> MESGIDLQGQFISALQSLGLSHDLAKLLWLPLPMLMMLIVATVGVLVAVWLERKISAAVQQRIGPEYIGPLGILAPLADGLKLIFKEDVLPANSDRWLFTLGPAVVVIPVFLSYIIVPFGQNLLISNLAMGVFLWIALSSIAPIGLLMAGYASNNKYSLLGGLRAAAQSISYEIPLALAVLAVAMMSNGLGTVEIVEQQSQYGILSWNVWRQPIGFLVFWIAALAECERLPFDLPEAEEELVAGYQTEYAGMKFALFYLGAYVNLVLSALLVSVLYFGGWSFPIPLETIANLLGVSETNPFLQIAFAVLGITMTLIKAYFFVFLAILLRWTVPRVRIDQLLDLGWKFLLPVGLVNLLLTAGLKLAFPVAFGG;> MDLVTLAGQLNAGTILPETILIVTLLVVLLADLIQGRQADRWTPYFAIVGLGGAIATMIPLWTQPATISFFGSFISDHLSLFFRGLIALSALGTILMSIRYVEQTGSSLGEFMTILLTATVGGMFIAGAQELVFIFVALETLSIASYLLTGYTKRDSRSNEAALKYLLIGAASSAIFLYGSSLLYGLSGGHTQLPAIAQALSSESLGLVVALVFVIAGISFKISAVPFHQWTPDVYEGAPTPVVAFLSVGSKAAGFALAIRFLTLAFPSVTDQWQLIFTVLAILSMILGNVVALAQTSMKRMLAYSSIGQAGFVMIGFVVGTEAGYASMLFYLLVYLFMNLGAFTCVILFSLRTGTDQISEYAGLYQKDPLLTLGLSLCLLSLGGIPPLAGFFGKIYLFWAGWQAGAYGLVLLGLLTSVISIYYYIRVVKMMVVKEPQEMSEAVRNYPEVSWSSFGLRPLQVGLVMTVIATSLAGILANPLFNLVNTAVWDVPQLANQPTVMEVAYQALSPAGKS;> MVAIPRLRDTATVFVLSGYEYFLGFLIICSLVPVLALAASALLRPKSGRMIRLTTYESGMEPIGGAWIQFNVRYYMFALVFVIFDVETVFLYPWAVAFHQLGLLAFIEALIFIAILVVALVYAWRKRALEWS;> MLHSLRFLPMLTLLIVLPVIGALLMPLLPERVLRSVALVIAGLTFALSLWMLTQFDVHQSALQFTEFVPWLLPLGLNYSLGVDGLSLPLIVLGTFLTLGVVFTGEKTGQRLFYALVLLANAGITGALAAQNLLLFFLFYELELVPFYLLILIWGGQRREQAAVKFLIYTAVSGILVLAAFLAMGWLTHAPSFDSADIQIAGLAPTTQGILLLLLILGFGIKMPLVPLHSWLPDAYVEASTPTAILLGGALAKLGAYGLVRFALGYFPEAWAQFSGLLAIVAAVGIAYGALAAIAQKDIKRMVAYSSIGHMSYVLLAAAAHTHLSMVGAIAQMISHGLILALLFYLVGVIETKVGTRELNVLNGLLNPLRGLPTTSALLILGGMASAGIPGLVGFVAEFLIFQGSYGMFPLPTLVAVVGTGLTAVYFVIMINRTCFGRLDNRTAYYPRVVWSEKMPALVLTLLIVFLGVQPTWLVRWSETTSAQIVAAVPRTNELVATLAKR;> MQLTYVLILAALLFCIGIYGLVTSRNAVRVLMSIELLLNAVNLNLIGFANYLDGQQIKGQVFAVFVITVAAAEAAVGLAIILAIYRNRDTVDMEKFNLLKW;> MLQSFADTVWLIPFYSLAGMVLSLIWSPGITRKTGPRPAGYLNILLTFFSFVHALLATVAIANQPPQYLHWTWLDVAGLHLDIPVEISILTTTALMLITALNLMAQVFAVGYMEMDWGWARFFALLALFEGGMGALVLLDSLFFNYVVLEILTLATYLLIGLWFNQPLVVTGARDAFLTKRVGDLVLLMGVLAIYPLAGSWNYDDLAAWAATAQVNSTLITLICLALIAGPMGKCAQFPLHLWLDEAMEGPIPASILRNAVVVATGAWVLVKLTPVLSLSPVALTALLVIGSVTALGGTLIAIAQVDIKRALSYLVSAYMGWVFIAVGLKEPGLAFVFILTYSLAMAVLMMSIGSIIWNSVTQDLRLLGGLWSRRPISGISFLVGSAGLLAVPPLASFFPQAELLDTAFAQLPWVGGVLLLMNTFAAFSLGRTFCLVWGGEVKPMTARSPEVFWPMILPMTVDLGLVLHLPILMARFDWVIWTQPSLATAAALTITALLGWGVAAWVYLGKAIPKPVQFPLPSVQNLLAYDFYTPKLYRATVVGVVDMISRITAWFDRTFVDGTGNAFGVVTLLGGDRLKYSTTGQSQAYILTILMGIAILVIAICWPLLA;> MDLATLTQTITFFALAAAVIIAALGVVLLDNVVYSAFLLGGVFLSIAGLYILMNADFVSAAQILIYVGAVNVLILFAIMLVNKRETYTPVPGRWLRQGGAAVVSLGVFALLTKMILQTPWQLSSVPPTPDSITTIGQHFFSDFLLPFELASVLLLMALIGAVVLARRELVLEPEPILGEEVVPPLELPERPREPVALSEK;> MPKIETRTEPMVINMGPHHPSMHGVLRLMVTLDGEDVIDCEPVIGYLHRGMEKIAENRTNIMFIPYVSRWDYAAGMFNEAVTVNAPEKLAGIPVPKRASYIRVIMLELNRIANHLLWLGPFLADVGAQTPFFYIFREREYIYDLFEAATGMRFINNNYFRIGGVAADLTYGWVTKCRDFCDYFLPKVDEYERLITNNPIFVRRLQGVGKISREEAINWGLSGPMLRASGVKWDLRKVDHYECYDDFDWDVPVATEGDCLARYIVRIQEMRESVKIIRQALDGLPGGPYENLEAKRMLEGAKSEWNGFDYQYIGKKLSPTFKIPKGEHYVRVESGKGELGIYLIGDDNVFPWRWKIRPPDFNNLQVLPQLLKGMKVADIVAILGSIDVIMGSVDR;> MKFLNQITNYAKEAVQSAKYIGQGLSVTFDHMRRRPITVQYPYEKLIPSERFRGRIHFEFDKCIACEVCVRVCPINLPVVDWVFNKELKKKELKHYSIDFGVCIFCANCVEYCPTNCLSVTEEYELATYDRHELNYDSVAMGRIPYKVTQDPMVTPIREFAYLPAGVMSGHDLPAGAQRAGERPEAIANTAKSSEN;> MSDTPEAPIVEAGPVGRLLQSQNLSVESLGRDASGVEMIKVDRDRLLAVCQTLYADGFNYLRCQAAYDSGPGQDLVSTYHLIKLSDNADRPPEVRIKVFVPRDDPRVPSVYWIWKTADWQERESYDMFGIVYEGHPNLKRILMPEDWVGWPLRKDYITPDFYELQEAY;> MTNTTSPAILNPIARPEVPQELAENIILTSLNDVYDWARLSSLWPLMYGTACCFIEFAAMIGSRFDFDRFGLVPRNSPRQADLIITSGTITMKMAPALVRLYEQMPSPKYVIAMGACTITGGMFSSDSYSAVRGVDKLIPVDVYLPGCPPRPEAIMDAIVKLRKKIANEHINERGNLAQTHRLFTAKHKMKPVPPILTGQYLNAPSRQAPPPALAAAMGIAVPALGEAVSETTSVAE;> MAVSTELLVLGVYGALAGLYLLVVPAIVYAYLNARWYVASSFERAFMYFLVTFFFPGLLLLAPFINFRPQPRSLNS;> MLLKSTTRHVHIYAGHVVDGEVHPDTETLTLNVDPDNELEWNEAALAKVEAKFRELVANAAGEDLTEYNLRRIGSDLEHFIRSLLMQGEIGYNLNSRVRNYSLGIPRVNHS;> MGLLAGYQFVKDLESAGALALFVPPEGGFEGRYQRRLRSKGYTTLPMSAPGLGDLAAYLTQEHGIRPAHTGKEDIRVYFQPPLVTYHLENLPPNAKGLVLWLIDGKRLSKQEFAYLAQLTQTLPKFKVVVEVGGDRVVRWEPLADWVAAA;> MAIKKGDLVKVVAEKLANSLEALASDHRYPPYLFEGRGEVVDIRGDYAQIKFPVPTPTVWLRLDQLEVAQ;> MVQAMERPSSAKLPPLDHPLADIIYRLEAGGALIPDTPVNLMKIIGMYKAYSIPMDFYWRDLLYLGERVFINPFPFFKYFPTKEYFELPNHYAGDTADLRIWRGPAHAHPELMEFIEKGETGKMPRLLHHLWHDRINMEFSEDLARAMMWHRMGGQLDIYLDSEEYKAAADKAIRAYFKRNPLMLGLYKLFPDLFLEQARQATYMNVLGLFWEVMAPVFFEISDRYDEGSITSVKDAMNFLVNGIFAIAGRPIYHHVYIDDEVHVLVPKEKGFMWLYEAAFPYVEAVFYRTSPFRGTKSYNAQANQVPTDQVDFHYGILFADKFPVGTAGIPPTLLHQDMYHFLPQYLKDYFHQHCRGEDDILVQLGIAFQHAMYTVTSAVLQATRAAFYYPLDDPNPEHLMANRRFFVAQMDRFLRPQYGIAEACKIRNVQDPNYL;> MATIVDIAVNTPGFSTLVTAVKVANLVEALQSPGPFTVFAPNDDAFAKLPDGTITSLVQNPPQLGRILKYHVVAGAYKATDLKRMGIVTSLEGSTIPIHGDNPLEVKNATVLAADIEAENGIIHVIDTVILMGLDPAHSFQETNIPYKV;> MIRPIADTYPLLPLSKAQMGQRQEIINSHKRLWDKTMATDLIMTILPGMTVKVTNPNDTYYQFQGIVQRITDGKVAVLFEGGNWDKLVTFQASELEPVVVTPKEKAKAKK

Cyanobacteria express instead the inducible NDH-1MS (NDH-13) and constitutive NDH-1MS’ (NDH-14) photosynthetic complex I isoforms that convert CO2 into HCO3− by kinetically shifting the reaction equilibrium towards bicarbonate, against high cytoplasmic HCO3− concentrations. The 0.5 MDa complex has an overall U-shape with 19 isolated subunits. The core structure is highly conserved across the complex I superfamily, but in contrast to the respiratory enzyme, the photosynthetic complex lacks the N-module that accepts electrons from nicotinamide adenine dinucleotide (NADH).

The catalytic site responsible for the CO2 chemistry in the 50 kDa CupA protein electrostatically binds NdhF3. CupA has a fold, comprising α-helices, which drastically differs from known carbonic anhydrases (CAs) in which the catalytic zinc (Zn2+) ion binds to histidine (αCA family) or histidine/cysteine residues (βCA family) at the interface of β-sheets. CupA is capped by the 16 kDa α-helical CupS subunit that binds two helical lobes of the former, and could help in stabilising the CupA-NdhF3 interaction. The active site of CupA shows a strong electron density that we assign to a Zn2+ ion, as also supported by inductively-coupled plasma optical emission spectrometry (ICP-OES), which indicates a protein-to-zinc ratio of ~0.7 in the NDH-1MS sample. The Zn2+ ion is coordinated by His130, a putative water/hydroxide ligand or carbonate, and Arg135. The Zn2+-site is located at the interface of two 12 Å helices, and CupA forms further contacts with NdhF3 and several lipid molecules. The putative CO2 binding pocket is completed by residues from NdhF3: the Zn2+-H2O/OH− is stabilised by Arg37 that forms an ion-pair with Glu114 and Tyr41 of NdhF3. A non-polar tunnel starting from NdhF3 that leads to the Zn2+-site via this Arg37/Glu114/Tyr41 network could function as a CO2 conduction channel from the luminal side across the membrane. Remarkably, NdhF3 binds a chlorophyll a/β-carotene motif that connects via His469 of NdhF3 in a TM-helix to the CupA site.>[4x]MWFGEFGGQYVPETLVGPLKELEKAYKRFKDDEEFNRQLNYYLKT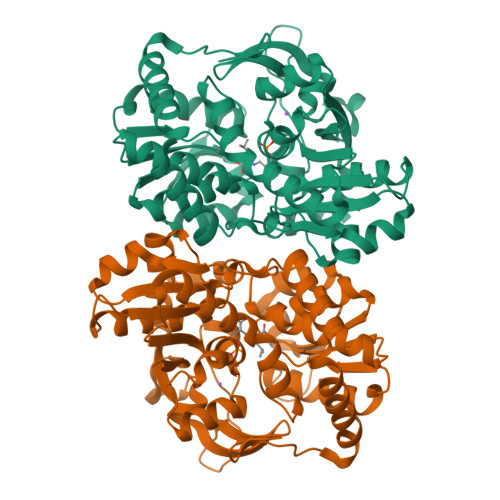WAGRPTPLYYAKRLTEKIGGAKIYLKREDLVHGGAHKTNNAIGQAPLAKLMGKTRLIAETGAGQHGVATAMAGALLGMKVDIYMGAEDVERQKMNVFRMKLLGANVIPVNSGSRTAKDAINEALRDWEATFEYTHYLIGSVVGPHPYPTIVRDFQSVIGREAKAQILEAEGQLPDVIVACVGGGSNAMGIFYPFVNDKKVKLVGVEAGGKGLESGKHSASLNAGQVGVLHGMLSYFLQDEEGQIKPSHSIAPGLDYPGVGPEHAYLKKIQRAEYVTVTDEEALKAFHELSRTEGIIPALESAHAVAYAMKLAKEMSRDEIIIVNLSGRGDKDLDIVLKASGNV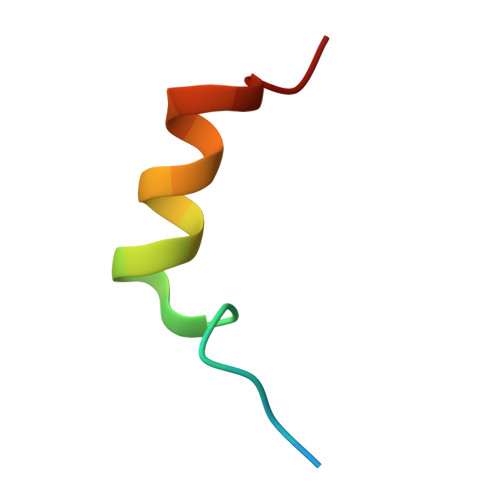> PTVVQSRTDVFNEQFANEALHPMT> MSGDEMIFDPTMSKKKKKKKKPFMLDEEGDTQTEET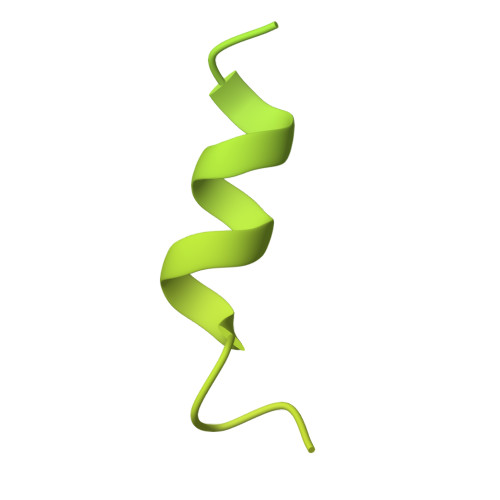QPSETKEVEPEPTEDKDLEADEEDTRKKDASDDLDDLNFFNQKKKKKKTKKIFDIDEAEEGVKDLKIESDVQEPTEPEDDLDIMLGNKKKKKKNVKFPDEDEILEKDEALEDEDNKKDDGISFSNQTGPAWAGSERDYTYEELLNRVFNIMREKNPDMVAGEKRKFVMKPPQVVRVGTKKTSFVNFTDICKLLHRQPKHLLAFLLAELGTSGSIDGNNQLVIKGRFQQKQIENVLRRYIKEYVTCHTCRSPDTILQKDTRLYFLQCETCHSRCSVASIKTGFQAVTGKRAQLRAKAN>QWIEPRNCARRYLKVDFADIGWSEWIISPKSFDAYYCSGACQFPMPKSLKPSNHATIQSIVRAVGVVPGIPEPCCVPEKMSSLSILFFDENKNVVLKVYPN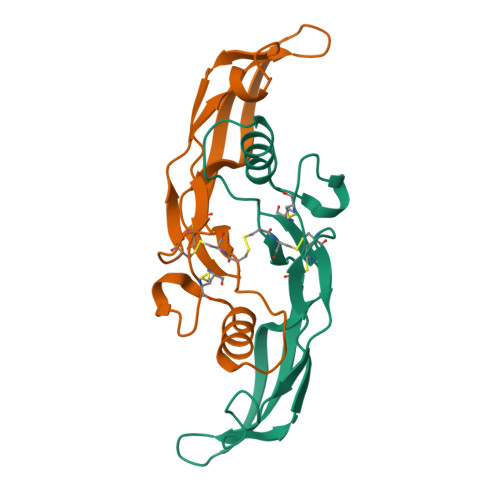MTVESCACR[2x]> MYLSKVIIARAWSRDLYQLHQGLWHLFPNRPDAARDFLFHVEKRNTPEGCHVLLQSAQMPVSTAVATVIKTKQVEFQLQVGVPLYFRLRA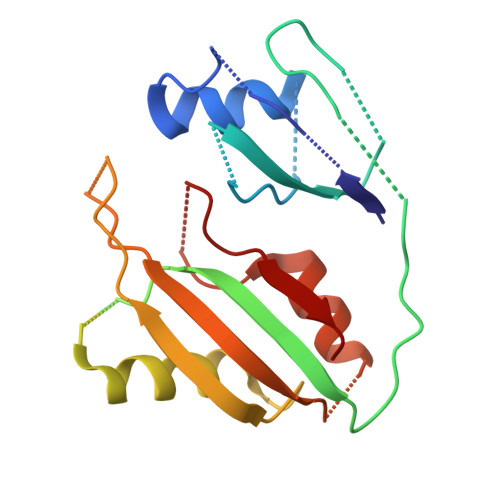NPIKTILDNQKRLDSKGNIKRCRVPLIKEAEQIAWLQRKLGNAARVEDVHPISERPQYFSGDGKSGKIQTVCFEGVLTINDAPALIDLVQQGIGPAKSMGCGLLSLAPL>MEKNMKFPVVDLSKLNGEERDQTMALINEACENWGFFEIVNHGLPHDLMDKIEKMTKDHYKTCQEQKFNDMLKSKGLDNLETEVEDVDWESTFYVRHL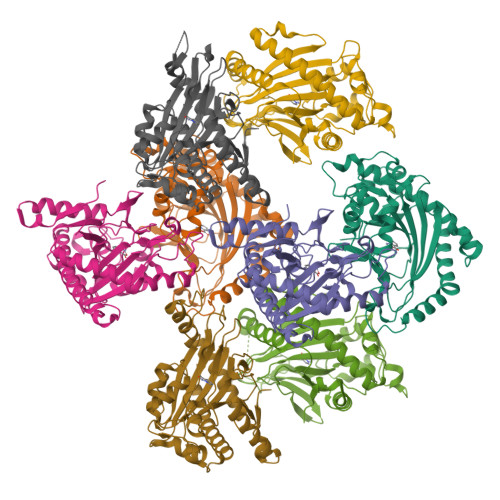PQSNLNDISDVSDEYRTAMKDFGKRLENLAEDLLDLLCENLGLEKGYLKKVFHGTKGPTFGTKVSNYPPCPKPEMIKGLRAHTDAGGIILLFQDDKVSGLQLLKDGDWIDVPPLNHSIVINLGDQLEVITNGKYKSVLHRVVTQQEGNRMSVASFYNPGSDAEISPATSLVEKDSEYPSFVFDDYMKLYAGVKFQPKEPRFAAMK[8x]>APTKVTFGDDTVIEVQGYKSVNITFELDERIDKVLNEKCSAYTVELGTEVNEFACVVADAVIKTL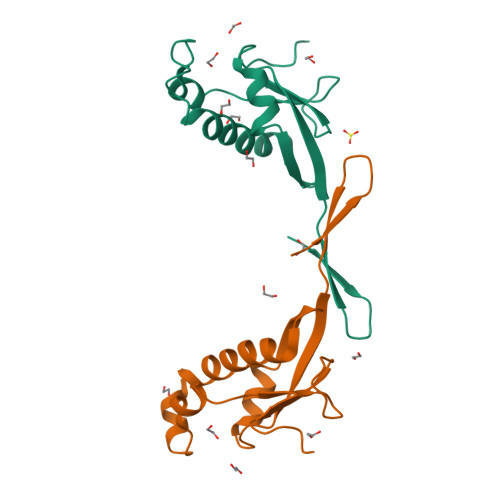QPVSELLTPLGIDLDEWSMATYYLFDESGEFKLASHMYCSFYPPDE[2x]(4~{S})-5-[2-chloranyl-4-[[3-chloranyl-4-(2-ethyl-2-oxidanyl-butoxy)phenyl]-dimethyl-silyl]phenoxy]-4-oxidanyl-pentanoic 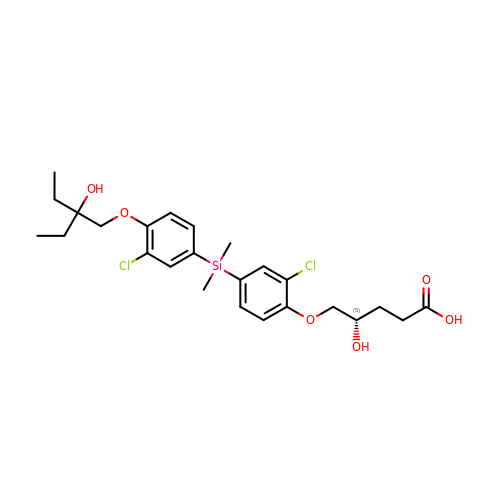acid | C25 H34 Cl2 O6 Si | WUCFPULJDHVZFU-KRWDZBQOSA-N> ATITQDTPINQIFTDTALAEKMKTVLGKTNVTDTVSQTDLDQVTTLQADRLGIKSIDGVEYLNNLTQINFSNNQLTDITPLKNLTKLVDILMNNNQIADITPLANLTNLTGLTLFNNQITDIDPLKNLTNLNRLELSSNTISDISALSGLTSLQQLSFSSNQVTDLKPLANLTTLERLDISSNKVSDISV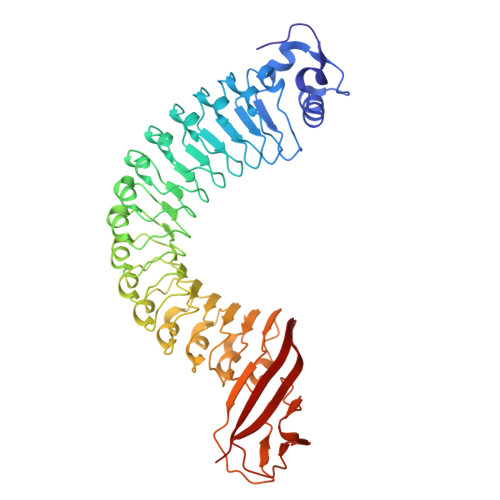LAKLTNLESLIATNNQISDITPLGILTNLDELSLNGNQLKDIGTLASLTNLTDLDLANNQISNLAPLSGLTKLTELKLGANQISNISPLAGLTALTNLELNENQLEDISPISNLKNLTYLTLYFNNISDISPVSSLTKLQRLFFYNNKVSDVSSLANLTNINWLSAGHNQISDLTPLANLTRITQLGLNDQAWTNAPVNYKANVSIPNTVKNVTGALIAPATISDGGSYTEPDITWNLPSYTNEVSYTFSQPVTIGKGTTTFSGTVTQPLKA>MSFPGWGPYPPVERDETSAITYSSKLHGSVTVRDPYSQLEVPFEDSEETKAFVHSQRKFARTYLDENPDREAWLETLKKSWNYRRFSALKPESDGHYYFEYNDGLQSQLSLYRVRMGEEDTVLTESGPGGELFFNPNLLSLDGNAALTGFVMSPCGNYWAYGVSEHGSDWMSIYVRKTSSPHLPSQERGKDPGRMNDKIRHVRFFIVSWTSDSKGFFYSRYPPEDDEGKGNAPAMNCMVYYHRIGEDQESDVLVHEDPEHPFWISSVQLTPSGRYILFAASRDASHTQLVKIADLHENDIGTNMKWKNLHDPWEARFTIVGDEGSKIYFMTNLKAKNYKVATFDANHPDEGLTTLIAEDPNAFLVSASIHAQDKLLLVYLRNASHEIHIRDLTTGKPLGRIFEDLLGQFMVSGRRQDNDIFVLFSSFLSPGTVYRYTFGEEKGYRSLFRAISIPGLNLDDFMTESVFYPSKDGTSVHM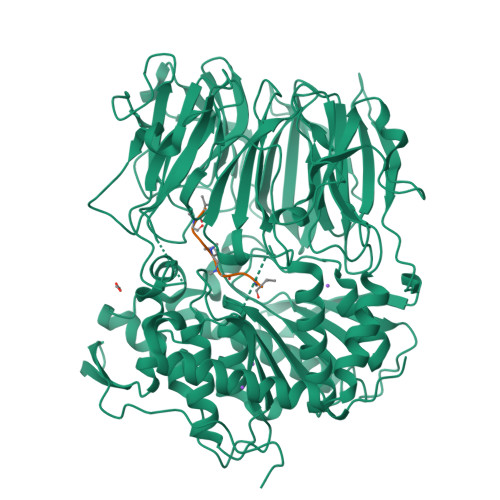FITRPKDVLLDGTSPVLQYGYGGFSLAMLPTFSLSTLLFCKIYRAIYAIPNIRGGSEYGESWHREGMLDKKQNVFDDFNAATEWLIANKYASKDRIAIRGGANGGVLTTACANQAPGLYRCVITIEGIIDMLRFPKFTFGASWRSEYGDPEDPEDFDFIFKYSPYHNIPPPGDTVMPAMLFFTAAYDDRVSPLHTFKHVAALQHNFPKGPNPCLMRIDLNSGHFAGKSTQEMLEETADEYSFIGKSMGLTMQTQGSVDSSRWSCVTV[4x];>WVIVVGVIGVIGSVMSTE[4x]>MQRRRFLAQAAGAAGAGLAAVGMPAMAQANPTVRWRMSTSWPKSLDTIYGSADELCKRVGQLTDGKFEIRAFPGGELVPSAQNMDAVSNGTVECNHVLSTMYIGKNTALTFDTGLSFGLNARQHNAWIHYGGGLQQLRELYKKYNIVNHVCGNVGVQMGGWYRKEIKSTADLNGLNM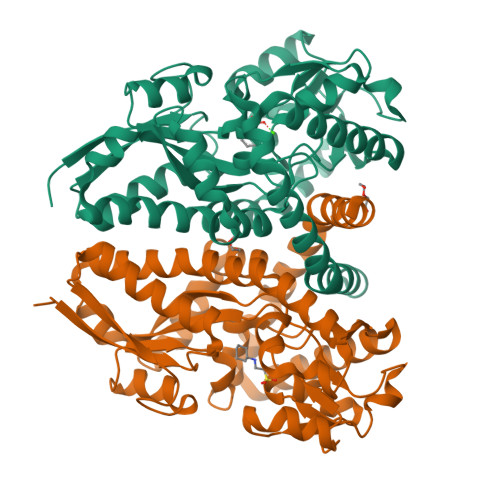RIGGIGGMVLSKLGVVPQQIPPGDIYPALEKGTIDAAEWIGPYDDEKLGFNKVAPYYYSPGWFEGSASITSMVNDKAWEALPPAYQAAFEAACGEQSMRMLANYDARNPLALRKLIAGGAKVSFFPKEVMDAVYKASQQLWTELSEKNPDFKAIYPGWKKFQEDEAGWFRVAENALDNYTFAAVARAQAK[2x]> PIFLNVLEAIEPGVVCAGHDNNQPDSFAALLSSLNELGERQLVHVVKWAKALPGFRNLHVDDQMAVIQYSWMGLMVFAMGWRSFTNVNSRMLYFAPDLVFNEYRMHKSRMYSQCVRMRHLSQEFGWLQITPQEFLCMKALLLFSIIPVDGLKNQKFFDELRMNYIKELDRIIACKRKNPTSCSRRFYQLTKLLDSVQPIARELHQFAFDLLIKSHMVSVD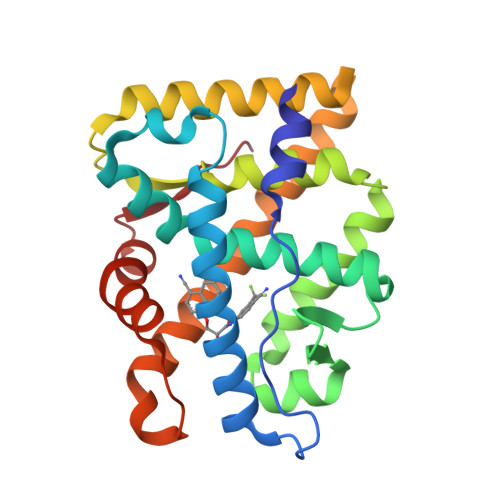FPEMMAEIISVQVPKILSGKVKPIYFH> TSSKIYDNKNQLIADL;> SNYPAYMDNYLKEVINQVEEETGYNLLTTGMDVYTNVDQEAQKHLWDIYNTDEYVAYPDDELQVASTIVDVSNGKVIAQLGARHQSSNVSFGINQAVETNRDWGSTMKPITDYAPALEYGVYESTATIVHDEPYNYPGTNTPVYNWDRGYFGNITLQYALQQSRNVPAVETLNKVGLNRAKTFLNGLGIDYPSIHYSNAISSNTTESDKKYGASSEKMAAAYAAFANGGTYYKPMYIHKVVFSDGSEKEFSNVGTRAMKETTAYMMTDMMKTVLTYGTGRNAYLAWLPQAGKTGTSNYTDEEIENHIKTSQFVAPDELFAGYTRKYSMAVWTGYSNRLTPLVGNGLTVAAKVYRSMMTYL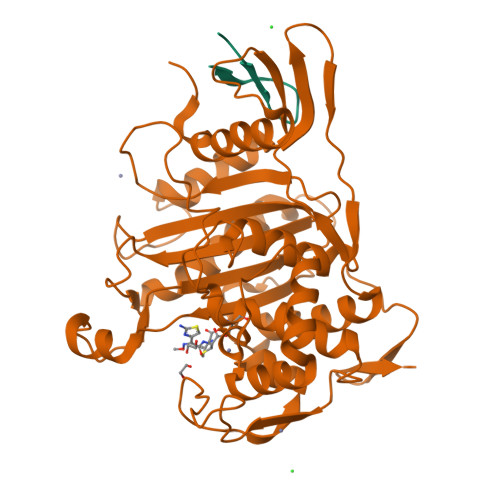SEGSNPEDWNIPEGLYRNGEFVFKN> MHHHHHHSSGRENLYFQGSTLSYTLGQLAAHVGAEVRGDADLPIQGLATLQEAGPAQLSFLANPQYRKYLPESRAGAVLLTAADADGFAGTALVVANPYLAYASLSHLFDRKPKAAAGIHPTAIVAADAEVDPSASVGAYAVIESGARIGAGVSIGAHCVIGARSVIGEGGWLAPRVTLYHDVTIGARVSIQSGAVIGGEGFGFANEKGVWQKIAQIGGVTIGDDVEIGANTTIDRGALSDTLIGNGVKLDNQIMIAHNVQIGDHTAMAACVGISGSAKIGRHCMLAGGVGLVGHIEICDNVFVTGMTMVTRSITEPGSYSSGTAMQPAAEWKKSAARIRQLDDMARRLQQLEKRLAAVTSSGD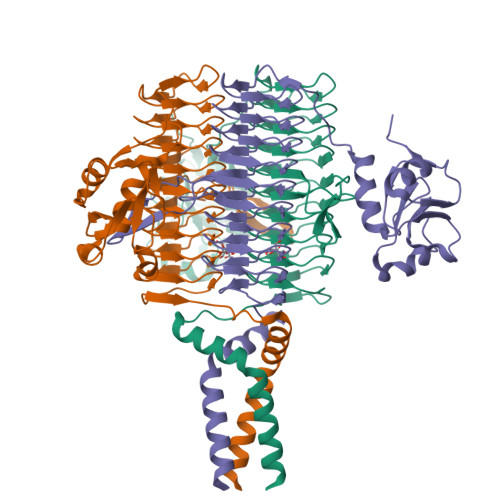ASSDA> MPKPAPRYNIGLRPAPKRQNVGGQFLATQKHYARELWYKRQYYSTRPFAIQKHMGSTPRILLDRTLWRSCWLTKSNLPDVNRWEKVVNSQRVTEDRWALVEEDGVMYQVN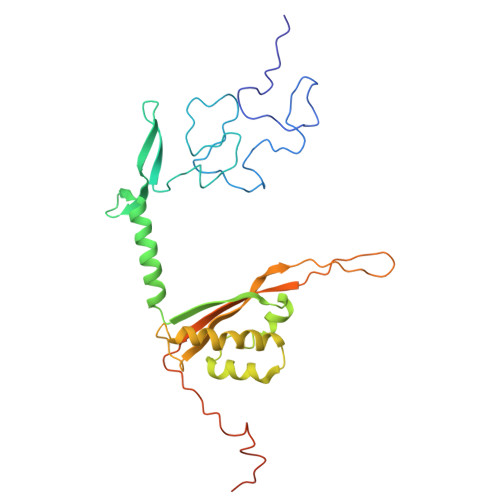WKMYCERLETELQKAQDQLPQYSFMMKAVPSAWKKLDIELSVLRGLSVREAMAQCKLSPRKGHMAVFRALEVAQQGAEGKGLDKEHLRIAYITCMPGPTDKQVDIRSRGYYAWKTKKSSHLLLTLAEDPEMVLPDRTAIPYASLMTMKRAGLRTEPTMLDVPAITAEGI We have determined high-resolution crystal structures of the ykkC guanidine III riboswitch from Thermobifida fusca. X-ray crystallography shows that the RNA folds into an H-type pseudoknot, in which a connecting strand locates in the major groove of one duplex to form a regular triple helix. This continues into the central core of conserved nucleotides that form a novel left-handed helical ramp of inter-nucleotide interactions, generating the guanidinium cation binding site. Comparison with earlier probing data suggest that the formation of the triple helix is stabilized by guanidine binding and this exposes the adjacent ribosome binding site to permit initiation of gene translation.

The majority of species crystallized in the trigonal space group P3121. The conformations were essentially identical in both crystal forms, with an all-atom root-mean-square deviation (RMSD) = 0.55 Å. Two of the guanidino nitrogen atoms are hydrogen bonded to O6 and N7 on the Hoogsteen edge of G7, while two are equivalently bonded to G17, so that one ligand nitrogen is hydrogen bonded to the O6 atoms of both G7 and G17 nucleobases. Lastly, we observe that the guanidine is stacked on the nucleobase of C6 at a distance of 3.5 Å. This is a π-cation interaction (Gallivan and Dougherty, 1999, Wintjens et al., 2000) between the positively charged guanidino cation and the aromatic nucleobase.

> CCGGACGAGGUGCGCCGUACCCGGUCACGACAAGACGGCGC>[4x]MKKLTSGPALPGKLADCTAQDLNRTELFLVEGDSAGGSAKQARDREYQAIMPLKGKILNTWEVSSDEVLASQEVHDISVAIGIDPDSDDLSQLRYGKICILADADSDGLHIATLLCALFVRHFRTLVKEGHVYVALPPLYRIDLGKEVYYALTEEEKTGVLEQLKRKKGKPNVQRFKGLGEMNPMQLRETTLDPNTRRLVQLVISD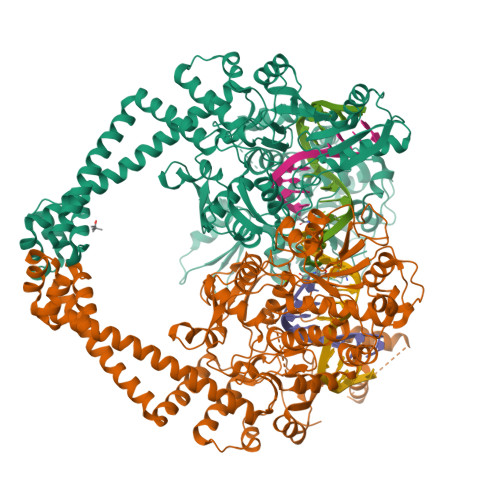EDEQQTTAIMDMLLAKKRSEDRRNWLQEKGDMADLEVEFMSDMAERLALHEFTENAYLNYSMYVIMDRALPFIGDGLKPVQRRIVYAMSELGLNASAKFKKSARTVGDVLGKYHPHGDSACYEAMVLMAQPFSYRYPLVDGQGNWGAPDDPKSFAAMRYTESRLSKYAELLLSELGQGTVDWVPNFDGTLQEPKMLPARLPNILLNGTTGIAVGMATDIPPHNLREVAKAAITLIEQPKTTLDELLDIVQGPDFPTEAEIITSRAEIRKIYQNGRGSVRMRAVWSKEDGAVVITALPHQVSGAKVLEQIAAQMRNKKLPMVDDLRDESDHENPTRLVIVPRSNRVDMEQVMNHLFATTDLEKSYRINLNMIGLDGRPAVKNLLEILSEWLVFRRDTVRRRLNHRLEKVLKRLHILEGLLVAFLNIDEVIEIIRTEDEPKPALMSRFGISETQAEAILELKLRHLAKLEEMKIRGEQSELEKERDQLQAILASERKMNNLLKKELQADADAFGDDRRSPLHEREEAKAMSLEHHHHHH> MSHHHHHHSGSMTQTDPAFQNLLAEFQALHAREPALAGFVALPDSLTPQPVTPV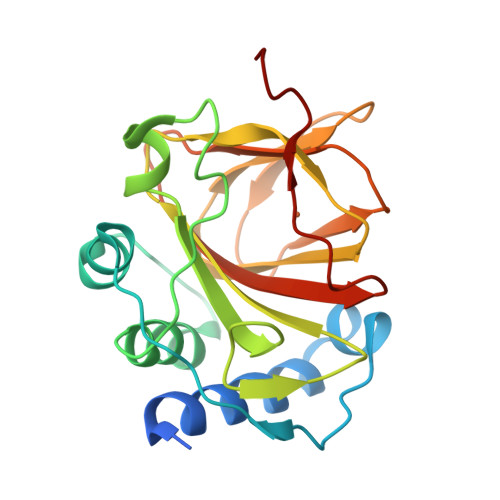RIPPAALMESDPDLTTTAYAAIRDAFIAAGAVAQWRLTYQGSRLGADFMDRFACYCLIGEGGPFASDSLAAYVVYMPAGLYYPFHQHPAEEIYFILAGEAEFLMEGHPPRRLGPGDHVFHPSGHPHATRTYDRPFMALVLWRGDLETAPVLTYPEGEI> MVTIMHIEELLDIEDHGERDRQLRRYLAPYSAEIGVDGAEKMALVVLLNLTLKRDRVESLCDEGLARQLLSDEGHITNCLHTVRWLHTHNLKYPDARVSGERLIINAPPLIPGVISSAGLPMRMGWAHDSSDINLAKLFGTSFRYRDDSTNLALQLVARSKTWEQALIGLGLTQQQLDIWCQLLASNLENNTFPTVVSPFSKQVRFLYQGNYCVVTPVVSHALLAQLQNVVHEKKLQCTYIHHDHPASVGSLVGALGGKVAVLDYPPPVSPDKARSFSQARKHRLANGQSLFDRSVFNDHVFIDALKHVISRPGLTRKQQRQLRLSALRYLRRQLAIWLGPIIEWRDEIVSSGRGEPGNLPSGGLELELITQPKKMLPELMLQVAGRFHLELQNHSAGRRFAFHPALMAPIKSQILWLLRQLADDEEKDEPHPPTSCYYLHLSGLTVYDASALANPYLCGIPSLSALAGFCHDYERRLQSLIGQSVYFRGLAWYLGRYSLVTGKHLPEPSKSADPKSVSAIRRPGLLDGRYCDLGMDLIIEVHIPTGGSLPFTTCLDLLRVALPARFAGGCLHPPSLYEEYNWCTVYQDKSTLFTVLSRLPRYGCWIYPSDADLRSFEELSEALALDRRLRPVATGFVFLEEPVERAGSIEGQHVYAESAIGTALCINPVEMRLAGKKRFFGAGFWQLNDAKGAILMNGSANTG;>[6x]MELCTHLSYSRSLSPGKAVFFYKTAESDFVPLRIEVAKISGQKCGYTEGFDANLKPKNIERYELAYSNPQTIEAC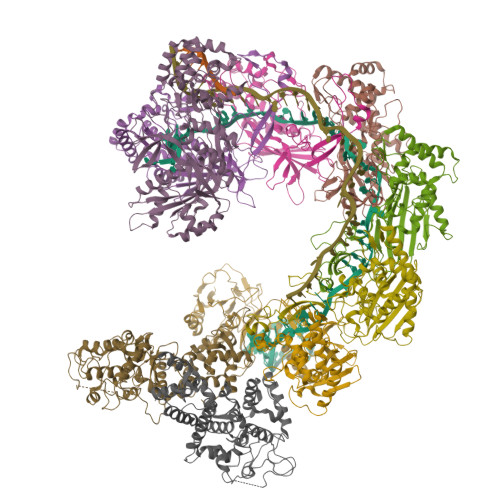YVPPNVDELYCRFSLRVEANSMRPYVCSNPDVLRVMIGLAQAYQRLGGYNELARRYSANVLRGIWLWRNQYTQGTKIEIKTSLGSTYHIPDARRLSWSGDWPELEQKQLEQLTSEMAKALSQPDIFWFADVTASLKTGFCQEIFPSQKFTERPDDHSVASRQLATVECSDGQLAACINPQKIGAALQKIDDWWANDADLPLRVHEYGANHEALTALRHPATGQDFYHLLTKAEQFVTVLESSEGGGVELPGEVHYLMAVLVKGGLFQKGKGR;> MTENRYFFAIRYLSDDVDCGLLAGRCISILHGFRQAHPGIQIGVAFPEWSDRDLGRSIAFVSTNKSLLERFRERSYFQVMQADNFFALSLVLEVPDTCQNVRFIRNQNLAKLFVGERRRRLARAKRRAKARGEAFQPHMPDETKVVGVFHSVFMQSASSGQSYILHIQKHRYERSEDSGYSSYGLASNDLYTGYVPDLGAIFSTLF;>MHLLVRPEPFADEALESYFLRLSQENGFERYRIFSGSVQDWLHTTDHAAAGAFPLELSRLNIFHASRSSGLRVRALQLVDRLTDGAPFRLLQLALCHSAISFGNHYKAVHRSGVDIPLSFIRVHQIPCCPDCLRESAYVRQCWHFKPYVGCHRHGGRLIYSCPACGESLNYLASESINHCQCGFDLRTASTVPAQPDEIQLSALAYGCSFESSNPLLAIGSLSARFGALYWYQQRYLSDHEAVRDDRALTKAIGHFTAWPDAFWRELQQMVDDALVRQTKPLNHTDFVDVFGSVVADCRQIPMRNTGQNFILKNLIGFLTDLVARHPQCRVANVGDLLLSAVDAATLLSTSVEQVRRLHHEGFLPLSIRPASRNTVSPHRAVFHLRHVVELRQARMQSHHDHSSTYLPAW[2x]>[3x]MESSKTEQVTGATGITQSTVTAPLPEAVSSLSLAPTVNALDPWVYLNQTEVPGGTFTVSSATQPGSVLLELEISPELNLYTSHLFRMYAGWSGGFSLKLLVAGNAFSAGKLIAAIIPPNIEVPNSAYLLTGFPHEILDFRTADSMEIIAPDIKNIDYHFRGDKLGKLVVMVYSPLRSTSADFEIEIKLTSAPLPDFKFTMLVPPIQNNALPIWSIPQAPPYSMVNPRSPLTPVVELYINSSYATCNHQLGRYTIYQGAIGNSTFNPSGAWTATCTAEAGSVTGHPNWRYALLDLPDNPTFDPTLPPVPRGFCDWGSGVKSGNKQHLVCFTGKKVEGGFQDVDTHMWDYGDNETVGLDNTYQRTIYIKDPSLEKDAQYLVIPMGVSGAANDDTVQVAPNCYGSWDYAPTVAPPLGEQFVWFRSQLPASKTTTTSGVNSVPVNVNALMSPDLMCSAYASGFPLGKVALLDYVLFGGSVVRQFKLYPEGYMTANTTGSNTGFIIPADGYFRFNSWVSPSFMISSVVDLNLQTAVVFR

Tulane virus (TV) has emerged as a crucial surrogate for HuNoVs due to its close resemblance in amino acid composition and the availability of a robust cell culture system. The structure of TV reveals the characteristic T = 3 icosahedral lattice comprising 90 dimers of the capsid protein VP1. VP1 subunits further divide into two domains: the shell domain (S domain), constituting the inner spherical shell of the virus capsid, and the protruding domain (P domain), further divided into the P1 and P2 sub-domains. In this study, we introduce, through cryo-electron microscopy (cryo-EM), the structure of a specific TV variant (the 9-6-17 TV) that has notably lost its ability to bind to its receptor, B-type HBGA—a finding confirmed using an enzyme-linked immunosorbent assay (ELISA).

To reduce this disulfide bond, we treated one sample with DTT and the other one without DTT to serve as the control sample. These two datasets used the same batch of viruses and were collected in the same session. The OptiPrep was largely dialyzed away for this sample. The identity of this extra density is unknown. Notably, four of these mutations are situated on the top surface of the P2 domain, which serves as the interaction surface with host cell receptors. An elongated extra density was found at the interface of the two subunits in both the A/B dimers and the C/C dimers near residues P425, V341 and M352. The pocket around it is mostly composed of hydrophobic residues (F329, V341, I380, M382, P425) with only one charged residue, D342, and one polar residue, T432.>[4x]ILVEGDGIPPPIKSFKEMKFPAAILRGLKKKGIHHPTPIQIQGIPTILSGRDMIG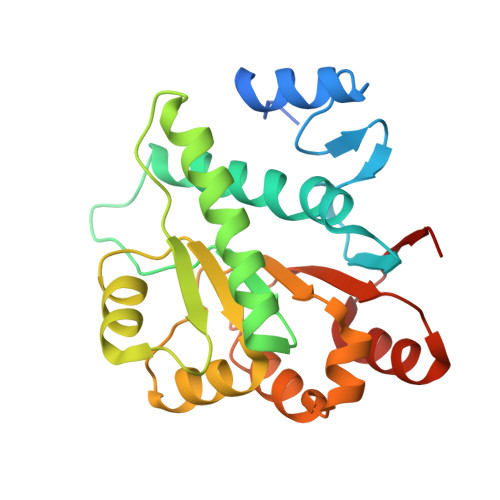IAFTGSGKTLVFTLPVIMFCLEQEKRLPFSKREGPYGLIICPSRELARQTHGILEYYCRLLQEDSSPLLRCALCIGGMSVKEQMETIRHGVHMMVATPGRLMDLLQKKMVSLDICRYLALDEADRMIDMGFEGDIRTIFSYFKGQRQTLLFSATMPKKIQNFAKSALVKPVTINVG>RGSHHHHHHTDPALRAITHISPLGSMDMLSQLEVDMLKRTASSDLYQLFRNCSLAVLNSGSLTDNSKELLSRFENFDINVLRRERGVKLELINPPEEAFVDGRIIRALQANLFAVLRDILFVYGQIHNTVRFPNLNLDNSVHITNLVFSILRNARALHVGEAPNMVVCWGGHSINENEYLYARRVGNQLGLRELNICTGCGPGAMEAPMKGAAVGHAQQRYKDSRFIGMTEPSIIAAEPPNPLVNELIIMPDIEK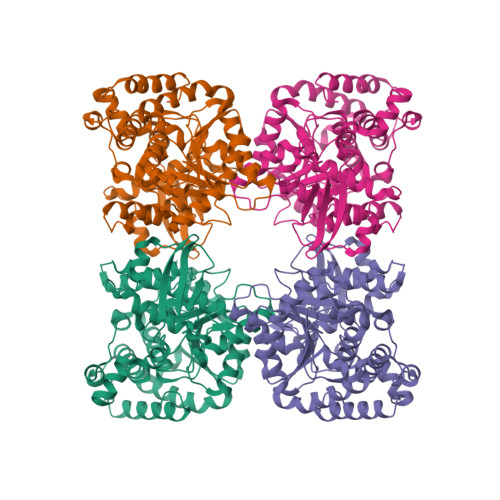RLEAFVRIAHGIIIFPGGVGTAEELLYLLGILMNPANKDQVLPLILTGPKESADYFRVLDEFVVHTLGENARRHYRIIIDDAAEVARQMKKSMPLVKENRRDTGDAYSFNWSMRIAPDLQMPFEPSHENMANLKLYPDQPVEVLAADLRRAFSGIVAGNVKEVGIRAIEEFGPYKINGDKEIMRRMDDLLQGFVAQHRMKLPGSAYIPCYEICTGLCGR[2x]>[2x]E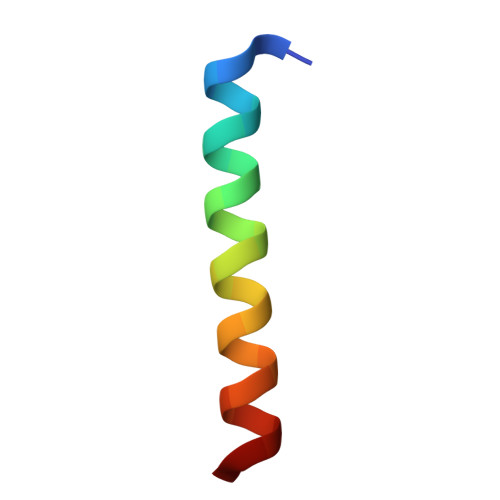ERKKELAKEVIETAKKLIEKLAKEE>MSTVEQVLEYVKSNNVKFMRFQFVDILGVPKNVAFPIKAGEKGIEELRDVLENGLYFDGSSIEGFVGINESDMMLKPDLSTFSVLPWRPSEKSVARVICDVYTTKGKPFEGDPRGCLKRVMEEFKKEFNGEYFVGPEPEFFLLKKDPHNPHKYIPADDGGYFDLEPMDEAPDIRRDIVFALENLGFHVEASHHEVAPGQHEVDFKFDDALKTADSVITFKTTIKTIAEQHGLKATFMPKPFFGMNGSGMHCHQSIWLNGEPSFYDENAPYQLSETCMNYVAGILKHAKAIVAITNPTVNSYKRLVPGYEAPVNIAWANSNRSAIIRVPAARGKGTRIEFRAPDPSCNPYLAFTVMLAAGLDGVKNKLDAPEPVERNIFAMSEAEKKELGIESVPANLKAALDELENNDVLKNALGKHIFESFLEIKNAEWDSFRTSVTDWETTAYLKI[6x]

Glutamine synthetases (GS) catalyze the ATP-dependent ammonium assimilation, the initial step of nitrogen acquisition that must be under tight control to fit cellular needs. The dodecamer is organized as two stacked hexameric rings, and each polypeptide is organized into two parts, a shorter N-terminal domain (β-Grasp fold) and the remaining C-terminal domain. The active sites are located at the interface of the N- and C- terminal domains of the adjacent subunit in the hexameric ring. Two loops in the active center are critical for catalysis: the Glu-flap, involved in shielding the active site during catalysis and deprotonating the intermediate product, and the Asp-50’ loop, which binds and deprotonates ammonium.

GS from Methanothermococcus thermolithotrophicus is inactive in its resting state and switched on by 2-oxoglutarate, a sensor of cellular nitrogen deficiency. The structure of MtGS in its resting state was solved by using the diffraction data obtained by Engilberge et al.. The data was collected on a crystal obtained by co-crystallization with a crystallophore (TbXo4) that corrected the twinning issue inherent to this crystalline form. The MtGS structure presents the typical homo-dodecameric architecture as seen in other structural homologs, with a monomeric unit divided into N-ter (1-111) and C-ter (112-448) domains. Moreover, terbium atoms are located in the active site, coordinated by the residues involved in the Mg2+/Mn2+ recognition. In the apo structure, water molecules replace 2OG in a pocket with a similar volume and slightly open to the solvent. In the resting state, the ATP would clash with the Phe206 and would not bind without displacing the β-sheet 10 (residues 199-205) and the following loop (206-209). In the resting state, the loop 318-325 is constrained by a network of hydrogen bonds and salt bridges from the Asp50ʹ-loop, the side chain of the Arg321 itself being sequestered by Glu70ʹ. In the resting state of MtGS without 2OG or the glutamine feedback-inhibited BsGS, the Glu-flap and the catalytic arginine are locked in an unproductive conformation by the Asp50ʹ-loop.> AVPKGKRSKHKCKQRQLIYFFDQFDGVFKRRRESFYRSFYNPP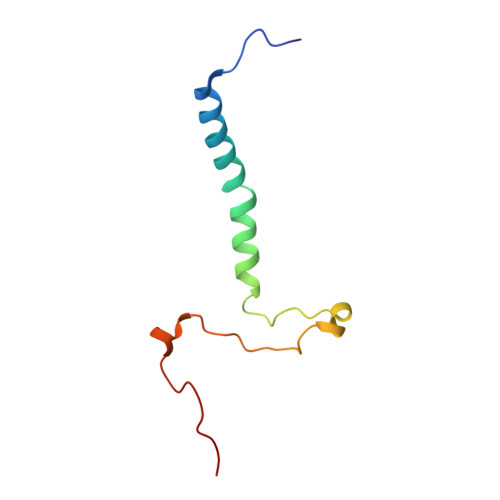YFSKQTEQTSLPPSVLRPFRFPGFWPGRFAFKMAS(2R,4S)-2-[(R)-carboxy{[(5-methyl-3-phenyl-1,2-oxazol-4-yl)carbonyl]amino}methyl]-5,5-dimethyl-1,3-thiazolidine-4-carboxylic acid | 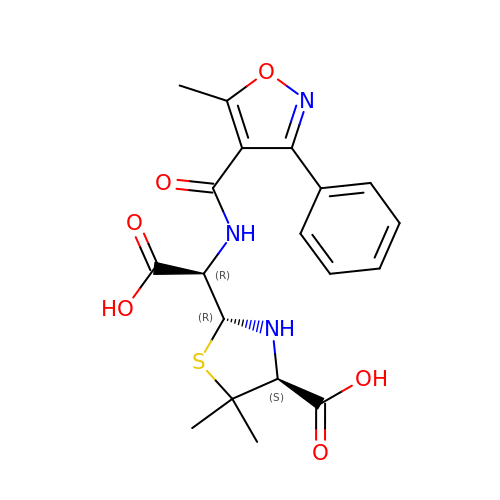C19 H21 N3 O6 S | JCHZLBSPYSDECZ-OFQRWUPVSA-N> XAKEWGYASHNGPEHWHELYPIAKGDNQSPIELHTKDIRHDPSLQPWSVSYDPGSAKTILNNGKTCRVVFDDTFDRSMLRGGPLSGPYRLRQFHLHWGSSDDHGSEHTVDGVKYAAELHLVHWNPKYNTFGEALKQPDGIAVVGIFLKIG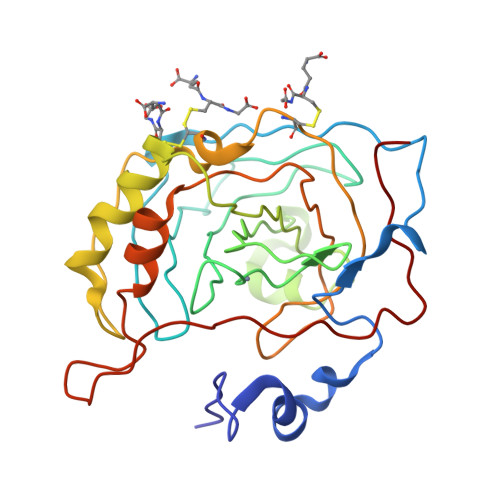REKGEFQILLDALDKIKTKGKEAPFNHFDPSCLFPACRDYWTYHGSFTTPPCEECIVWLLLKEPMTVSSDQMAKLRSLFASAENEPPVPLVGNWRPPQPIKGRVVRASFK> XPWSHP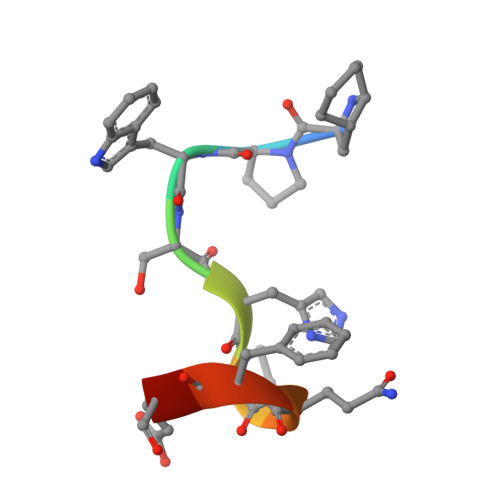QFEK> GPLGSSIMKILLIGDSGVGKSCLLVRFVEDKFNPSFITTIGIDFKIKTVDINGKKVKLQLWDTAGQERFRTITTAYYRGAMGIILVYDVTDERTFTNIKQWFKTVNEHANDEAQLLLVGNKSDM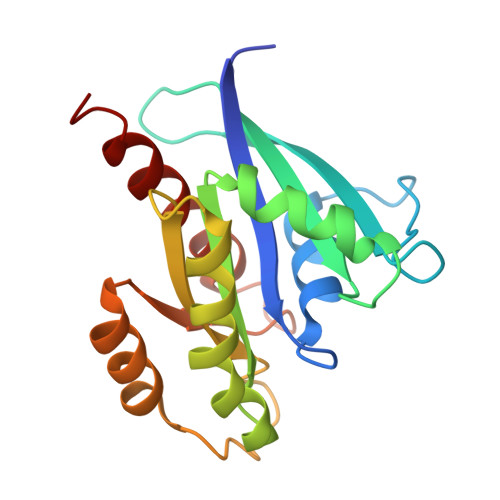ETRVVTADQGEALAKELGIPFIESSAKNDDNVNEIFFTLAKLIQEKIDSN> GPLGSMPGIDKLPIEETLEDSPQTRSLLGVFEEDATAISNYMNQLYQAMHRIYDAQNELSAATHLT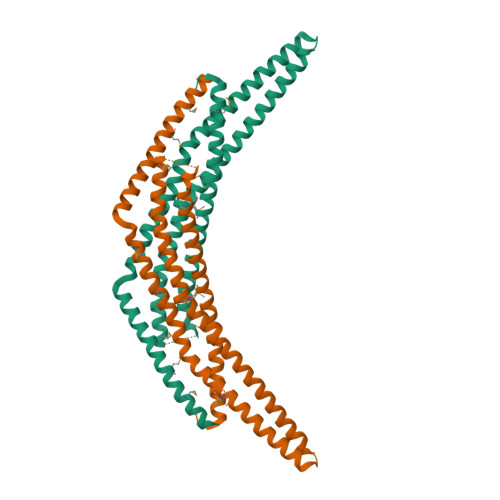SKLLKEYEKQRFPLGGDDEVMSSTLQQFSKVIDELSSCHAVLSTQLADAMMFPITQFKERDLKEILTLKEVFQIASNDHDAAINRYSRLSKKRENDKVKYEVTEDVYTSRKKQHQTMMHYFCALNTLQYKKKIALLEPLLGYMQAQISFFKMGSENLNEQLEEFLANIGTSVQNVRREMDSDIETMQQTIEDLEVASDPLYVPDPDPTKFPVNR>MKGGAGVPDLPSLDASGVRLAIVASSWHGKICDALLDGARKVAAGCGLDDPTVVRVLGAIEIPVVAQELARNHDAVVALGVVIRGQTPHFDYVCDAVTQGLTRVSLDSSTPIANGVLTTNTEEQALDRAGLPTSAEDK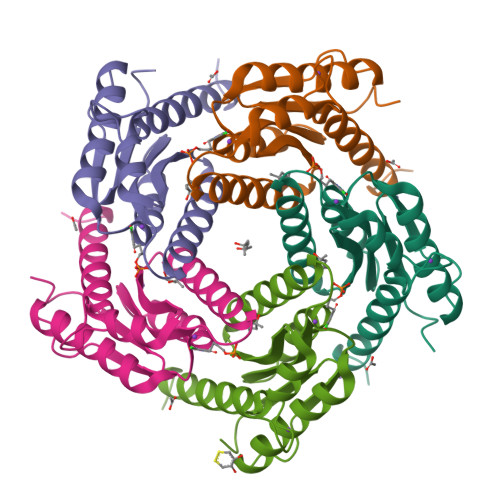GAQATVAALATALTLRELRAHS[5x]PHOSPHORYLISOPROPANE | C3 H9 O4 P | 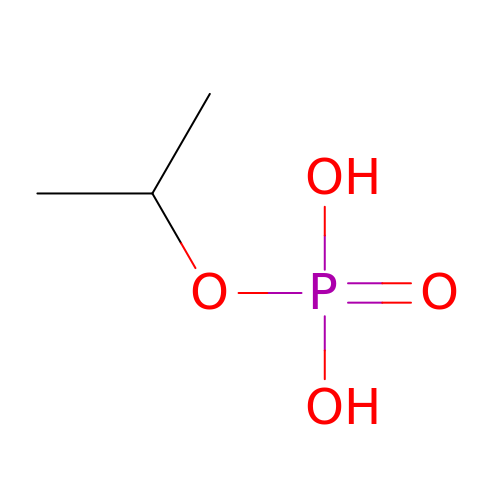QPPQHRDVPBTVEV-UHFFFAOYSA-N> RADVKPVTVKLVDSQATMETRSLFAFMQEQRRHSIMFGHQHETTQGLTITRTDGTQSDTFNAVGDFAAVYGWDTLSIVAPKAAGDIVAQVKKAYARGGIITVSSHFDNPKTDTQKGVWPVGTSWDQTPAVVDSLPGGAYNPVLNGYLDQVAEWANNLKDEQGRLIPVIFRLYHENTGSWFWWGDKQSTPEQYKQLFRYSVEYLRDVKGVRNFLYAYSPNNFWDVTEANYLERYPGDEW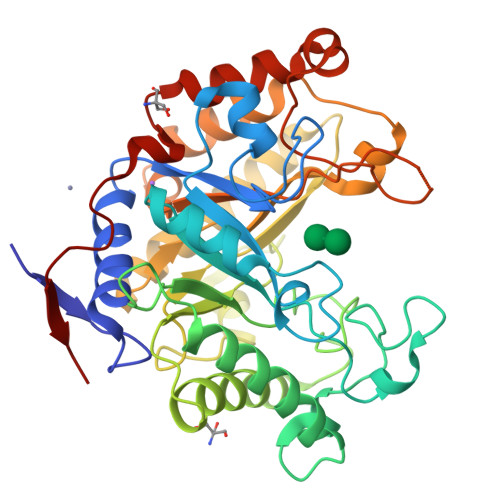VDVLGFDTYGPVADNADWFRNVVANAALVARMAEARGKIPVISGIGIRAPDIEAGLYDNQWYRKLISGLKADPDAREIAFLLVWRNAPQGVPGPNGTQVPHYWVPANRPENINNGTLEDFQAFYADEFTAFNRDIEQVYQRPTLIVK> GSHMKNPYSNQIEREELILKYLPLVKAIATNIKKHLPEDVDIRDLISYGVIGLIKAVDNLSTENPKRAEAYIKLRIKGAIYDYLR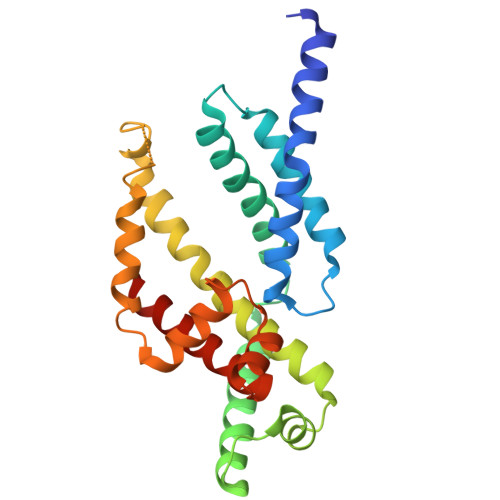SLDFGSRQVREKERRIKEVVEKLKEKLGREPTDEEVAKELGISTEELFKTLDKINFSYILSLEEVFRDFARDYSELIPSSTNVEEEVIKRELTEKVKEAVSKLPEREKLVIQLIFYEELPAKEVAKILETSVSRVSQLKAKALERLREMLSNPL>[6x]SNATHHQVLNGNTVSRQEIRLGLPSKGRMSSDTLDLLKDCQLSVKQVNPRQYVAQIPQISNLEVWFQRPKDIVRKLLSGDLDLGIVGLDVLTEFGQGNEDL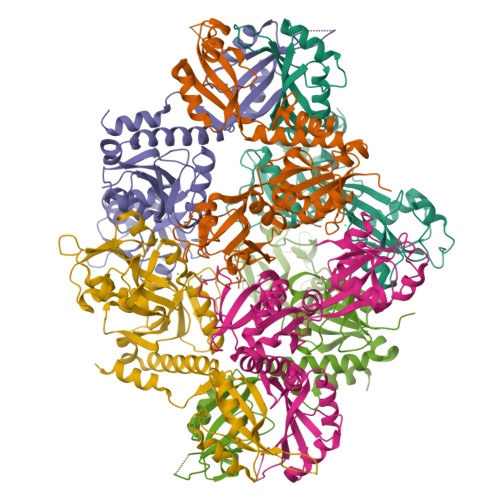IVVHEALEYGDCRLSIAIPQYGIFENVNSLEELAKMPQWTEDKPLRVATGFTYLGPKFMKDNGIKHVAFSTADGALEAAPAMGIADAILDLVSSGTTLKENNLKEIEGGTVLESQAALVASRRSMIGRKGVLETTHEMLERLEAHLRAMGQFTVVANMRGSSAEEVAERVLSQPSLAGLQGPTVSPVFCKRDGKVSADYYAIVICVPKKALYKSIQQLRAIGGSGVLVSPLTYIFDEETPRWRQLLSKLGL>[6x]MHHHHHHARATGKTFRSGNSEAVRLPRDLAFGADVELTLIRSGDVLTIYPSKGSIADLVATLNQMPRPDSVEIRDEDL;>MAYVLDTNV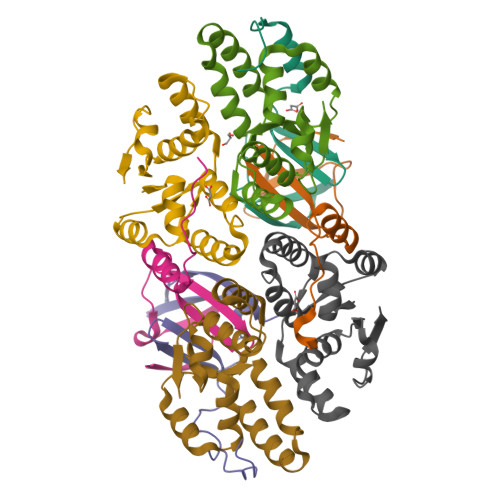AIHLRDGDPEVTTRVTALNGAILLSIISRVELEGGVYREAAQAGLRRSRLDVMLKVLPVLDFDGAAADEYRRIVESAGYSRRKVVDRMIAAQALAHRATFVTFNADDFRDIPGLSLLAW[6x]> GAESLTVAATPVPHAEILNVVKPLLAKEGVDLKIKEFTDYVQPNVQVSEKRLDANFFQHQPYLDEFNKAKGTDLVAVTGVHIEPLGAYSSKYKKLDELPSGATVVIPNDATNGGRALLLLDKAGVIKLKDNKSITATPKDIVDNPKNIKIRELEAATLPRVLTQVDMALINTNYALEAKLNPTKDALAIEGSDSPYVNILVARPDNKDSDAM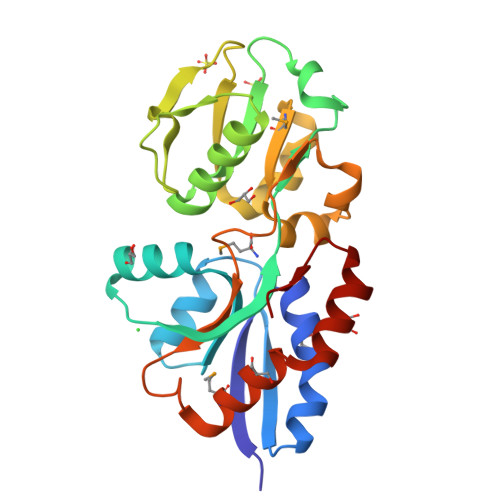QKLAKALHSAEIKQFIQEKYKGAVVPAF> SLTRIDHIGIACHDLDATVEFYRATYGFEVFHTEVNEEQGVREAMLKINDTSDGGASYLAL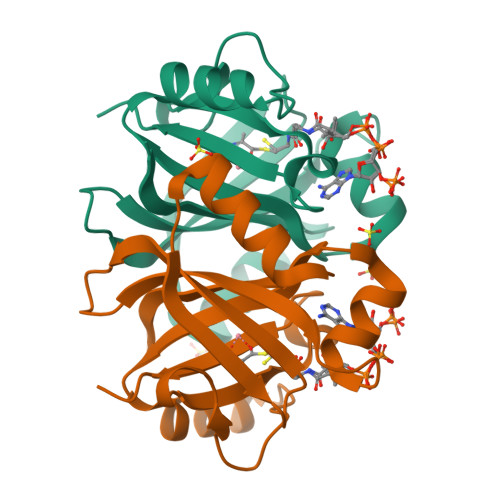LEPTREDSAVGKWLAKNGEGVHHIAFGTADVDADAADIRDKGVRVLYDEPRRGSMGSRITFLHPKDCHGVLTELVTSAAVESPEH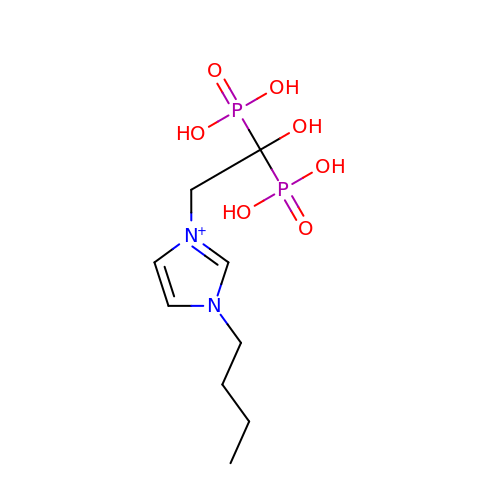1-butyl-3-(2-hydroxy-2,2-diphosphonoethyl)-1H-imidazol-3-ium | C9 H19 N2 O7 P2 | JCMWHMYRNYPQAZ-UHFFFAOYSA-O CYCLOTRIDECYL 3,4,6-TRIDEOXY-3-(DIMETHYLAMINO)-BETA-D-XYLO-HEXOPYRANOSIDE 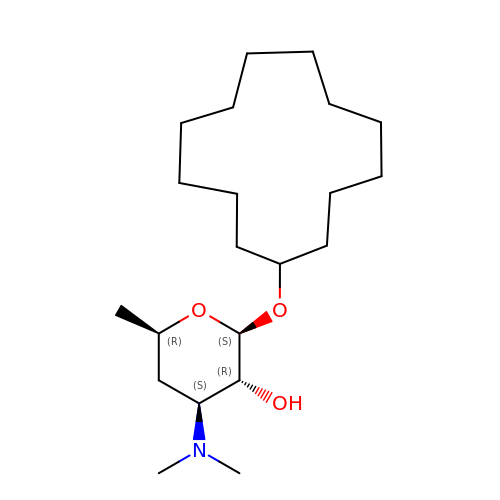| C21 H41 N O3 | LWQXCAWVTFBYID-PMXSJFBMSA-N N-[4-methyl-3-(1H-1,2,4-triazol-5-yl)thiophen-2-yl]-2-(2-oxo-3,4-dihydroquinolin-1(2H)-yl)acetamide | C18 H17 N5 O2 S | 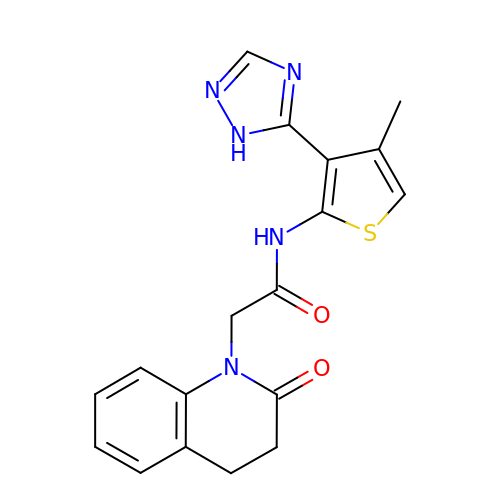HJUDFJRTVGXBRF-UHFFFAOYSA-N> FNLDAEAPAVLSGPPGSFFGFSVEFYRPGTDGVSVLVGAPKANTSQPGVLQGGAVYLCPWGASPTQCTPIEFDSKGSRLLESSLSSSEGEEPVEYKSLQWFGATVRAHGSSILACAPLYSWRTEKEPLSDPVGTCYLSTDNFTRILEYAPCRSDFSWAAGQGYCQGGFSAEFTKTGRVVLGGPGSYFWQGQILSATQEQIAESYYPEYLINLVQGQLQTRQASSIYDDSYLGYSVAVGEFSGDDTEDFVAGVPKGNLTYGYVTILNGSDIRSLYNFSGEQMASYFGYAVAATDVNGDGLDDLLVGAPLLMDRTPDGRPQEVGRVYVYLQHPAGIEPTPTLTLTGHDEFGRFGSSLTPLGDLDQDGYNDVAIGAPFGGETQQGVVFVFPGGPGGLGSKPSQVLQPLWAASHTPDFFGSALRGGRDLDGNGYPDLIVGSFGVDKAVVYRGRPVV;> QTDENRCLKANAKSCGECIQAGPNCGWCT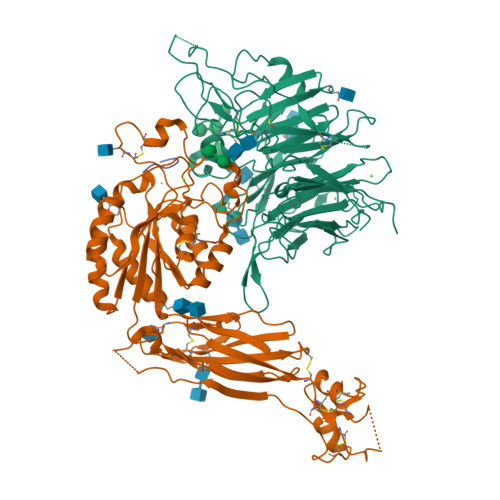NSTFLQEGMPTSARCDDLEALKKKGCPPDDIENPRGSKDIKKNKNVTNRSKGTAEKLKPEDITQIQPQQLVLRLRSGEPQTFTLKFKRAEDYPIDLYYLMDLSYSMKDDLENVKSLGTDLMNEMRRITSDFRIGFGSFVEKTVMPYISTTPAKLRNPCTSEQNCTTPFSYKNVLSLTNKGEVFNELVGKQRISGNLDSPEGGFDAIMQVAVCGSLIGWRNVTRLLVFSTDAGFHFAGDGKLGGIVLPNDGQCHLENNMYTMSHYYDYPSIAHLVQKLSENNIQTIFAVTEEFQPVYKELKNLIPKSAVGTLSANSSNVIQLIIDAYNSLSSEVILENGKLSEGVTISYKSYCKNGVNGTGENGRKCSNISIGDEVQFEISITSNKCPKKDSDSFKIRPLGFTEEVEVILQYICECE;> GRGDSP>[4x]GSHMSEEAKIAIELFKEAMKDPERFKEMCSPDT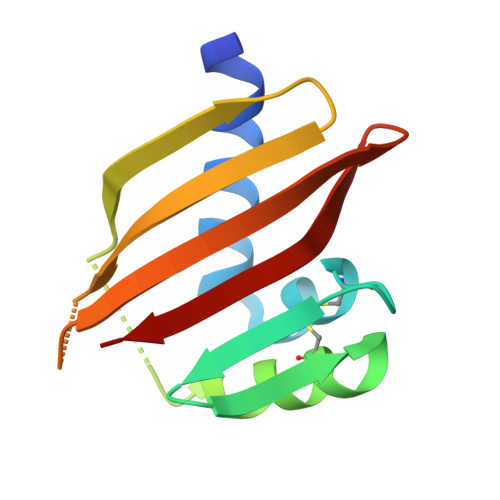RIESNGQEYRGSEECKKFAEEMKKTHPWEVRVERYRSDGDRFEIELRVNFNGKTFRMEIRMRKVNGEFRIEEMRLHG> ATDAASLVGELQALDAEYQNLANQEEAR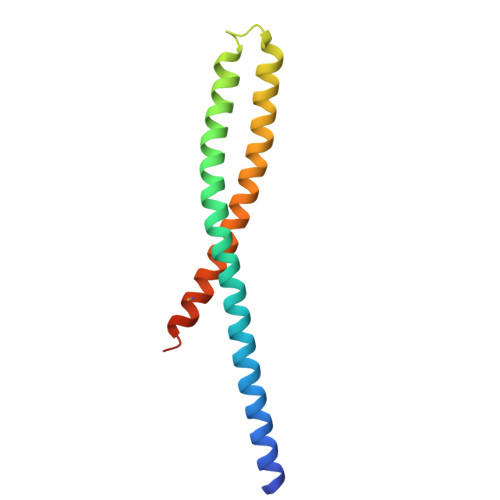FNEERAQADAARQALAQNEQVYNELSQRAQRLQAEANTRFYKSQYQELASKYEDALKKLEAEMEQQKAVISDFEKIQALRAGNLEHHHHHH> GAMDYSLVKALQTAQQNFVISDPSIPDNPIVYASQGFLTLTGYALSEVLGRNCRFLQGPETDPKAVEKVRKGLERGEDTTVVL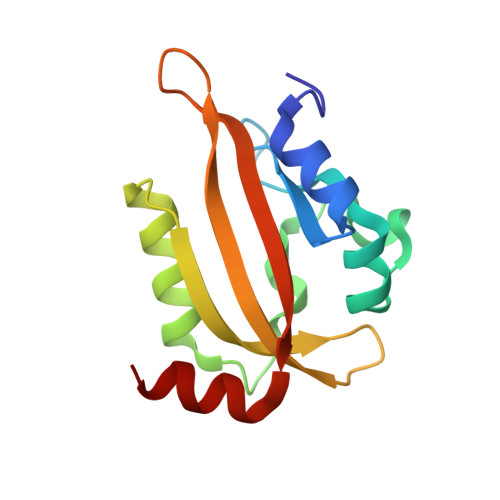LNYRKDGSTFWNQLFIAALRDGEGNVVNYLGVQCKVSEDYAKAFLKN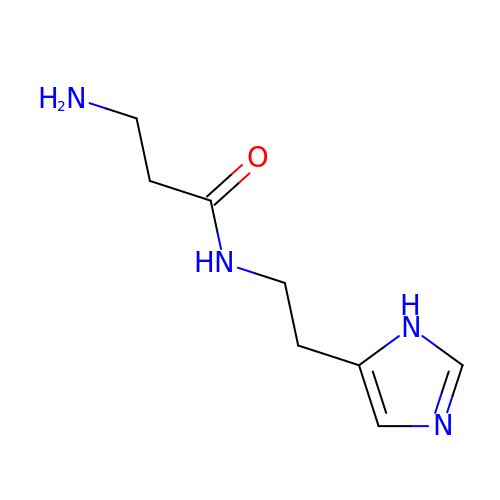N-[2-(1H-imidazol-5-yl)ethyl]-beta-alaninamide | C8 H14 N4 O | ANRUJJLGVODXIK-UHFFFAOYSA-N(2S)-2-chloranyl-2-[(2R)-5-oxidanylidene-2H-furan-2-yl]ethanoic 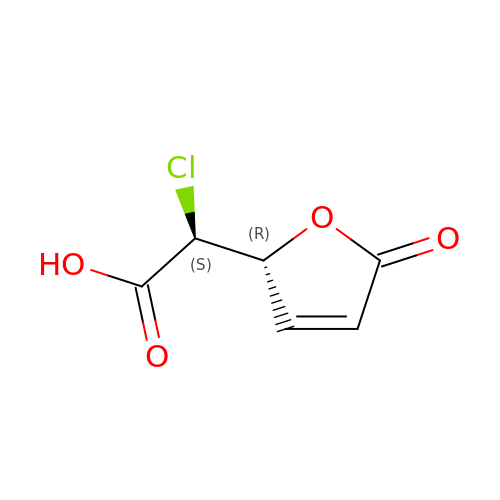acid | C6 H5 Cl O4 | KGCZGOVWTWDEQD-WUJLRWPWSA-N> LEEAPWPPPEGAFVGFVLSRKEPMWADLLALAAARGGRVHRAPEPYKALRDLKEARGLLAKDLSVLALREGLGLPPGDDPMLLAYLLDPSNTTPEGVARRYGGEWTEEAGERAALSERLFANLWGRLEGEERLLWLYREVERPLSAVLAHMEATGVRLDVAYLRALSLEVAEEIARLEAEVFRLAGHPFNLNSRDQLERVLFDELGLPAIGKTEKTGKRSTSAAVLEALREAHPIVEKILQYRELTKLKSTYIDPLPDLIHPRTGRLHTRFNQTATATGRLSSSDPNLQNIPVRTPLGQRIRRAFIAEEGWLLVALDYSQIELRVLAHLSGDENLIRVFQEGRDIHTETASWMFGVPREAVDPLMRRAAKTINFGVLYGMSAHRLSQELAIPYEEAQAFIERYFQSFPKVRAWIEKTLEEGRRRGYVETLFGRRRYVPDLEARVKSVREAAERMAFNMPVQGTAADLMKLAMVKLFPRLEEMGARMLLQVHDELVLEAPKERAEAVARLAKEVMEGVYPLAVPLEVEV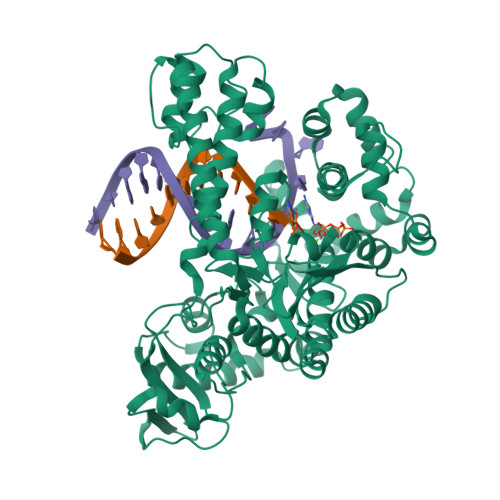GIGEDWLSAKE> SSSNYCNQMMKSRNLTKDRCKPVNTFVHESLADVQ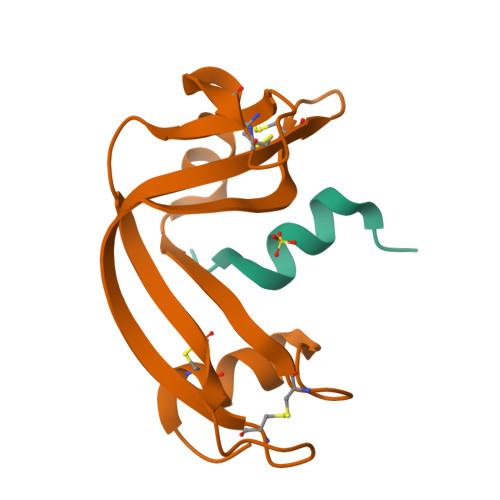AVCSQKNVACKNGQTNCYQSYSTMSITDCRETGSSKYPNCAYKTTQANKHIIVACEGNPYVPVHFDASV;> KETAAAKFERQHGDSX>MIVADSECRAELKDYLRFAPGGVGDSGPGEEQRESRARRGPRGPSAFIPVEEVLREGAESLEQHLGLEALMSSGRVDNLAVVMGLHPDYFTSFWRLHYLLLHTDGPLASSWRHYIAIMAAARHQCSYLVGSHMAEFLQTGGDPEWLLGLHRAPEKLRKLSEINKLLAHRPWLITKEHIQALLKTGEHTWSLAELIQALVLLTHCHSLSSFVFGCGILPEGDADGSPAPQAPTPPSEQSSPPSRDPLNNSGGFESARDVEALMERMQQLQESLLRDEGTSQEEMESRFELEKSESLLVTPSADILEPSPHPDMLCFVEDPTFGYEDFTRRGAQAPPTFRAQDYTWEDHGYSLIQRLYPEGGQLLDEKFQAAYSLTYNTIAMHSGVDTSVLRRAIWNYIHCVFGIRYDDYDYGEVNQLLERNLKVYIKTVACYPEKTTRRMYNLFWRHFRHSEKVHVNLLLLEARMQAALLYALRAITRYM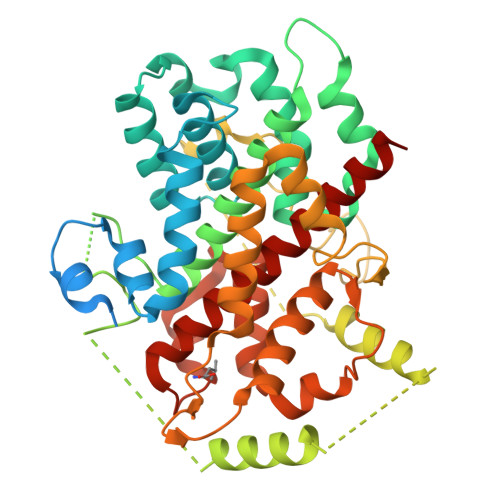T[5x]> MSVKESLSLLNSMQGNVKIGNVEPAKGNEGYVDNAGYVDCTKSYFEATKSLKEEQLVCDPKFTLLDSISAFEIMEPKMDSGIDYQPLRVDFSRDLSYLEILALMDLIVSAEKEWHYGSPLSESLLCSAHVFSICKSPISQVGDSGFSSGSGRNTTDIVLFPFVLAVIKCCDIVHREFLMGNLYDEEDISSFSYHMSFLQNYPIEKLNYLLQSSIEYLASEVIKFSAELRQIIEGILNRIQLR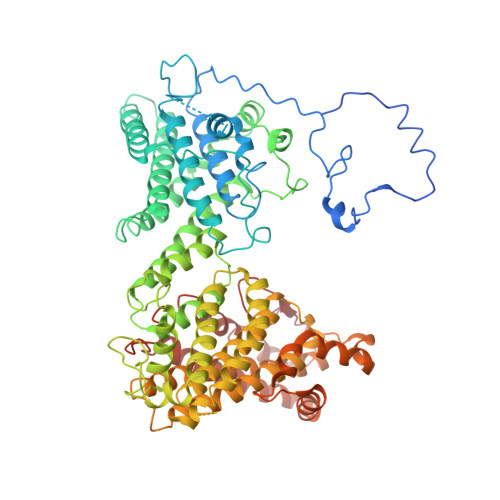IGILRVYERSDIKTTIDALHLIKNLVPEIQNTVSVVDSSIKESILKQYWDFRVQAQLVATAPVRNIPPTGIEHSYQRILYFADDMLLILNSHTLASSLAVYQFCLDFTRLNRTPEPYVRSSLQALITANNAVNLRDQPTSYMLECIREFSGLPSNFYNPNTRTVIEKNSISSAYGPLVESLIAHSTNIMVDLVRICSHNPCRFRRNLINLLPEITVAHFEAEALDLKFVAKSLPSNGPFSSFIYHVKLNAIEHILLSSFEQKLHQPYQWPHFFAVLDHVFSIHQTHLELHGKDRNTPPMAKTFVTYLHRILNAIKETYSGYLLLTVLCMRLNIIKTPSFTLDEKIQESYYMAHYRPLINLRQPKPLLRSEADCIIKNLQNFSTDDLIIKSNEKFTAAKNSLINVIKSGFEQNEFINPYFLQTNYLKNLLCCCITNLVSLAILSKDHSANLKIVEIPGNPLPSLSRT> MSEEAFIYEAIRTPRGKQKNGSLHEVKPLSLVVGLIDELRKRHPDLDENLISDVILGCVSPVGDQGGDIARAAVLASGMPVTSGGVQLNRFAASGLEAVNTAAQKVRSGWDDLVLAGGVESMSRVPMGSDGGAMGLDPATNYDVMFVPQSIGADLIATIEGFSREDVDAYALRSQQKAAEAW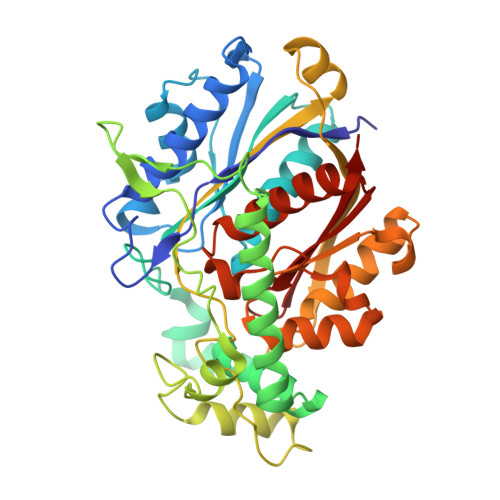SGGYFAKSVVPVRDQNGLLILDHDEHMRPDTTKEGLAKLKPAFEGLAALGGFDDVALQKYHWVEKINHVHTGGNSSGIVDGAALVMIGSAAAGKLQGLTPRARIVATATSGADPVIMLTGPTPATRKVLDRAGLTVDDIDLFELNEAFASVVLKFQKDLNIPDEKLNVNGGAIAMGHPLGATGAMILGTMVDELERRNARRALITLCIGGGMGVATIIERV> MSALPEEVNRTLLQIVQAFASPDNQIRSVAEKALSEEWITENNIEYLLTFLAEQAAFSQDTTVAALSAVLFRKLALKAPITHIRKEVLAQIRSSLLKGFLSERADSIRHKLSDAIAECVQDDLPAWPELLQALIESLKSGNPNFRESSFRILTTVPYLITAVDINSILPIFQSGFTDASDNVKIAAVTAFVGYFKQLPKSEWSKLGILLPSLLNSLPRFLDDGKDDALASVFESLIELVELAPKLFKD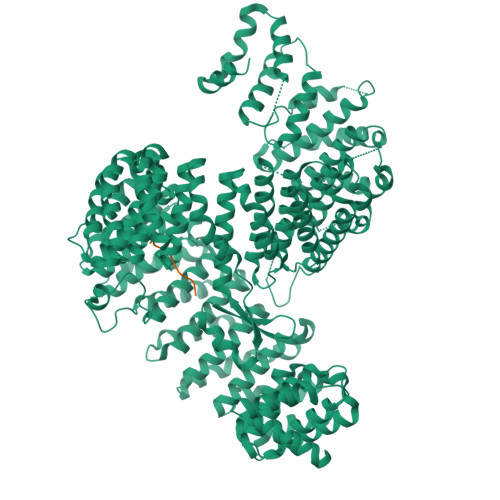MFDQIIQFTDMVIKNKDLEPPARTTALELLTVFSENAPQMCKSNQNYGQTLVMVTLIMMTEVSIDDDDAAEWIESDDTDDEEEVTYDHARQALDRVALKLGGEYLAAPLFQYLQQMITSTEWRERFAAMMALSSAAEGCADVLIGEIPKILDMVIPLINDPHPRVQYGCCNVLGQISTDFSPFIQRTAHDRILPALISKLTSECTSRVQTHAAAALVNFSEFASKDILEPYLDSLLTNLLVLLQSNKLYVQEQALTTIAFIAEAAKNKFIKYYDTLMPLLLNVLKVNNKDNSVLKGKCMECATLIGFAVGKEKFHEHSQELISILVALQNSDIDEDDALRSYLEQSWSRICRILGDDFVPLLPIVIPPLLITAKATQDVGLIEEEEAANFQQYPDWDVVQVQGKHIAIHTSVLDDKVSAMELLQSYATLLRGQFAVYVKEVMEEIALPSLDFYLHDGVRAAGATLIPILLSCLLAATGTQNEELVLLWHKASSKLIGGLMSEPMPEITQVYHNSLVNGIKVMGDNCLSEDQLAAFTKGVSANLTDTYERMQDRHGDGDEYNENIDEEEDFTDEDLLDEINKSIAAVLKTTNGHYLKNLENIWPMINTFLLDNEPILVIFALVVIGDLIQYGGEQTASMKNAFIPKVTECLISPDARIRQAASYIIGVCAQYAPSTYADVCIPTLDTLVQIVDFPGSKLEENRSSTENASAAIAKILYAYNSNIPNVDTYTANWFKTLPTITDKEAASFNYQFLSQLIENNSPIVCAQSNISAVVDSVIQALNERSLTEREGQTVISSVKKLLGFLPSSDAMAIFNRYPADIMEKVHKWFA;> RNAEFKVSKNSTSFKNPRRLEIKDGRSLFLRNRGKIHSGVLSSIESDL>[2x]MAKKDEVGGRVLQDVFLDWAKKYGPVVRVNVFHKTSVIVTSPESVKKFLMSTKYNKDSKMYRALQTVFGERLFGQGLVSECNYERWHKQRRVIDLAFSRSSLVSLMETFNEKAEQLVEILEAKADGQTPVSMQDMLTYTAMDILAKAAFGMETSMLLGAQKPLSQAVKLMLEGITASRNTLAKFLPGKRKQLREVRES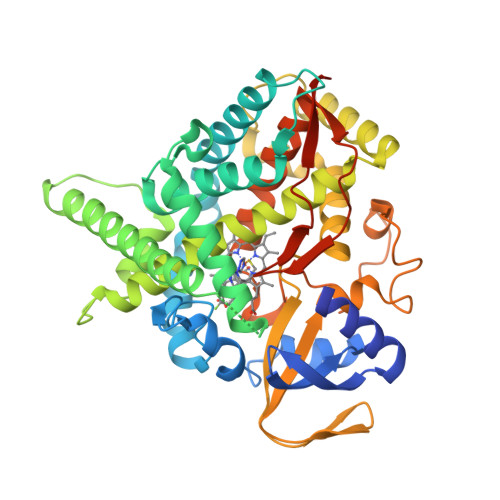IRFLRQVGRDWVQRRREALKRGEEVPADILTQILKAEEGAQDDEGLLDNFVTFFIAGHETSANHLAFTVMELSRQPEIVARLQAEVDEVIGSKRYLDFEDLGRLQYLSQVLKESLRLYPPAWGTFRLLEEETLIDGVRVPGNTPLLFSTYVMGRMDTYFEDPLTFNPDRFGPGAPKPRFTYFPFSLGHRSCIGQQFAQMEVKVVMAKLLQRLEFRLVPGQRFGLQEQATLKPLDPVLCTLRPRGWQPAPPPPPCHHHH Aggregation-prone-motifs (APRs) of proteins are short segments, which – as isolated peptides - form diverse amyloid-like crystals. We introduce two APRs - designed variants of the incretin mimetic Exendin-4 - that both display crystal-phase polymorphism. Crystallographic and spectroscopic analysis revealed that a single amino-acid substitution can greatly reduce topological variability: while LYIQWL can form both parallel and anti-parallel β-sheets, LYIQNL selects only the former. We found that a simple change in crystallization temperature or modest changes of chemical composition of the solvent system (therefore the available interaction partners) can prompt formation of significantly different nanostructures: we identified four different polymorphs of the LYIQWL and two of the LYIQNL APR peptides.

Needle-like crystals grew from 0.1 M acetate buffer, both in the presence and absence of ethanol at pH=4.8 and diffracted to a resolution of 1.70 Å and 1.55 Å, respectively. Crystals grown from both solvents contained β-strands of parallel orientation, but arranged in different amyloid topologies. In the monoclinic crystals grown from the ethanol containing solvent system, strands arranged in the class 3 topology could be observed, while the orthorhombic crystals grown in the absence of ethanol contained strands arranged according to the class 4 topology. Similarly to the class 3 structure, hydrophobic residues (Leu and Ile) form a hydrophobic niche in this arrangement too, while polar side chains of Asn and Gln stabilize the interface enforced by H-bonds. The side chain of Tyr2 forms H-bonds with chain termini. Due to the parallel orientation of the β-strands, Tyr ladders with a distance of 4.8 Å between adjacent side chains are formed in both crystal structures. On the other hand, in the class 4 arrangement, the Tyr side chains face in the same direction, so that inter-β-sheet Tyr-Tyr interactions could not form at the zipper interface. Although the Tyr side chains also meet near the chain ends in this crystal form, the interplanar distance between them is 7.0 Å, indicating a much weaker, if any, type of interaction. While the class 4 structure did not contain any solvent molecules, the class 3 structure contained both water molecules and two ethanol molecules, one in a solvent channel near the chain termini and another wedged into the steric zipper interface. The two polymorphic structures with distinctly different topologies are thereby stabilized by very similar interaction patterns.

> LYIQNL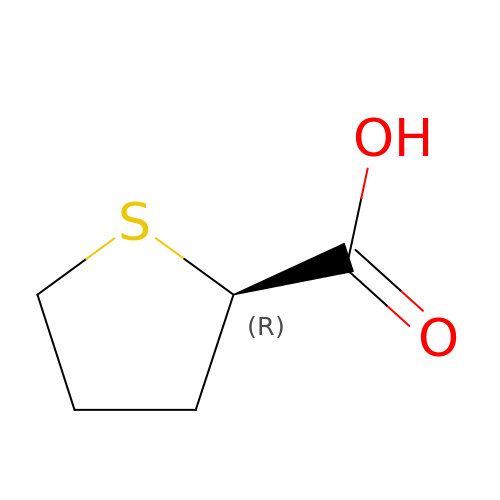(2R)-thiolane-2-carboxylic acid | C5 H8 O2 S | MZOYMQRKTJRHGJ-SCSAIBSYSA-N> F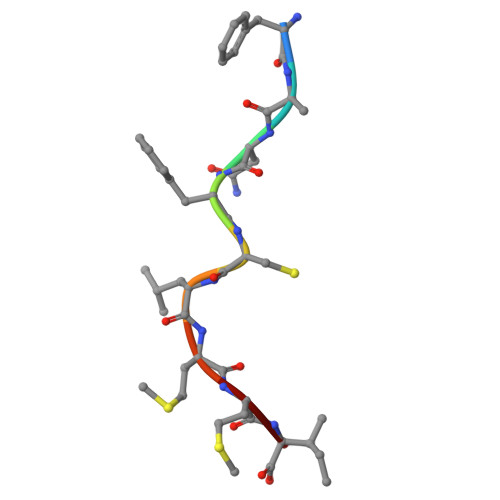ANFCLMMI> DYKDDDDKLVPRGSCHPRLSLHRPALEDLLLGSEANLTCTLTGLRDASGATFTWTPSSGKSAVQGPPERDLCGCYSVSSVLPGCAQPWNHGETFTCTAAHPELKTPLTANITKSGNTFR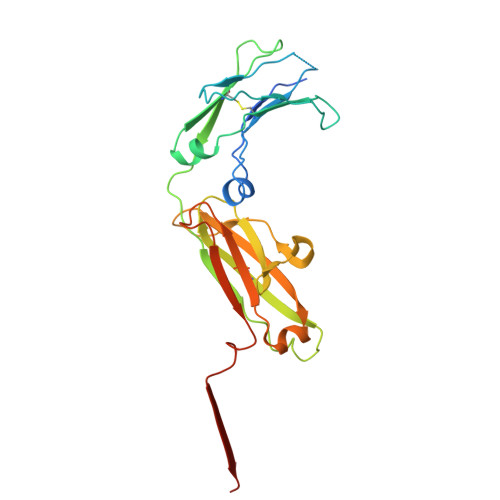PEVHLLPPPSEELALNELVTLTCLARGFSPKDVLVRWLQGSQELPREKYLTWASRQEPSQGTTTYAVTSILRVAAEDWKKGETFSCMVGHEALPLAFTQKTIDRLAGKPTHINVSVVMAEADGTCY> MGMLNAWHLPVPPFVKQSKDQLLITLWLTGEDPPQRIMLRTEHDNEEMSVPMHKQRSQPQPGVTAWRAAIDLSSGQPRRRYSFKLLWHDRQRWFTPQGFSRMPPARLEQFAVDVPDIGPQWAADQIFYQIFPDRFARSLPREAEQDHVYYHHAAGQEIILRDWDEPVTAQAGGSTFYGGDLDGISEKLPYLKKLGVTALYLNPVFKAPSVHKYDTEDYRHVDPQFGGDGALLRLRHNTQQLG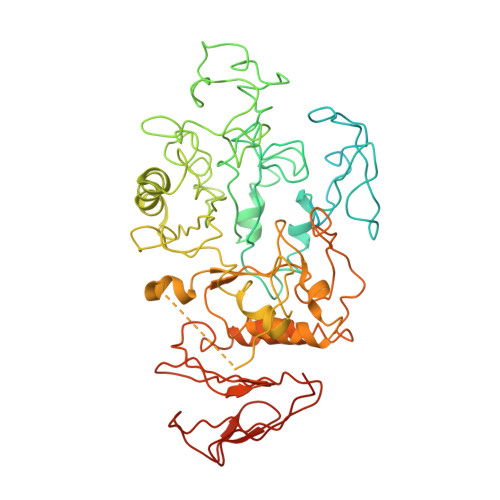MRLVLDGVFNHSGDSHAWFDRHNRGTGGACHNPESPWRDWYSFSDDGTALDWLGYASLPKLDYQSESLVNEIYRGEDSIVRHWLKAPWNMDGWRLDVVHMLGEAGGARNNMQHVAGITEAAKETQPEAYIVGEHFGDARQWLQADVEDAAMNYRGFTFPLWGFLANTDISYDPQQIDAQTCMAWMDNYRAGLSHQQQLRMFNQLDSHDTARFKTLLGRDIARLPLAVVWLFTWPGVPCIYYGDEVGLDGKNDPFCRKPFPWQVEKQDTALFALYQRMIALRKKSQALRHGGCQVLYAEDNVVVFVRVLNQQRVLVAINRGEACEVVLPASPFLNAVQWQCKEGHGQLTDGILALPAISATVWMNGSRSHHHHHH> SNAMLILSTEKEPNFEYEEITRSFLSNMLAFTRGHFTGDISHFSPIVLAEMEKDPNWLEE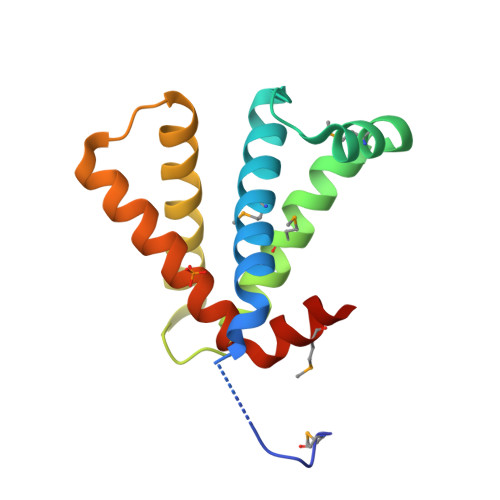AAGGMQGVIVQSLLEDENFSSVEQLKGELARLIRLYFALAKDNLTENQESLYVDLFDKFTFLLLCSDEFIMYLDSQPKF> ENKCIAVNENKVIENQKVIQSLCKNSHLDLIEQSYFGECDFIINHSTCVYKIQASRFMQLRNNGSLHYDKAVNDLLTEFQRVIIIVEFSEIIQDVDPDLFWKIKLYLLNSRVDVFFIHETTDFFIDWMKYFIARWAFSY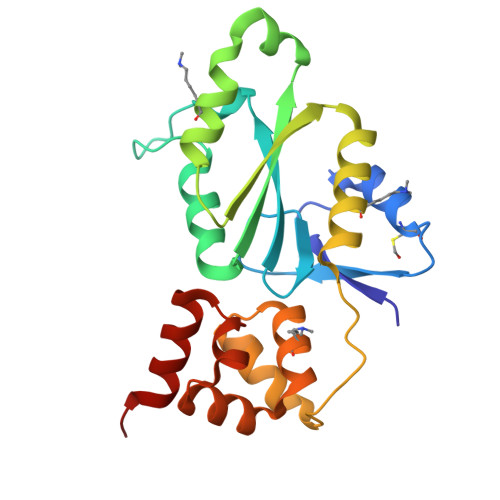NDEKEKNIANADILLDLGFNILLVRKIFQTYSLEEFFMAIIKEESKAVKMLTVSQMTRLKKLLTLEW>GHHHHHHHSTASSKITAAPMVYVRGEEMTAYVMDLIRSRWIEPRVDVGGWETFDLRAKNRDDTEDRVLRDVIEAGKRIKAIFKEPTVTPTADQVKRLGLRKSWGSPNGAMRRGWNGITISRDTIHIDGVELGYKKPVLFERHAVGGEYSAGYKNVGKGKLTTTFTPSEGPDAGKTVVVDEREIVDEEAAVVTYHNPYDNVHDLARFFFGRCLEAKVTPYVVTKKTVFKWQEPFWQIMRTVFDEEFKAQFVAAGVMKEGEELVHLLSDAATMKLVQWRQGGFGMAAHNYDGDVLTDELAQVHKSPGFITSNLVGVHEDGTLIKEFEASHGTVADMDEARLRGEETSLNPLGMVEGLIGAMNHAADVHNIDRDRTHAFTTKMRTVIHQLFRE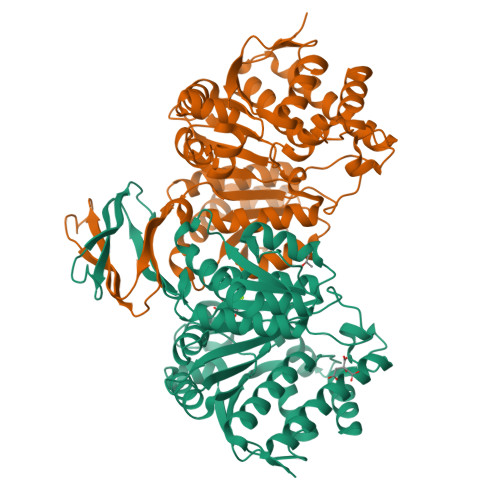GKGTRDLCGPSGLTTEQFIDAVAERLDA[4x]> GAMGSGEPQSPSRRVFNPYTEFKEFSRKQIKDMEKMFKQYDAGRDGFIDLMELKLMMEKLGAPQTHLGLKNMIKEVDEDFD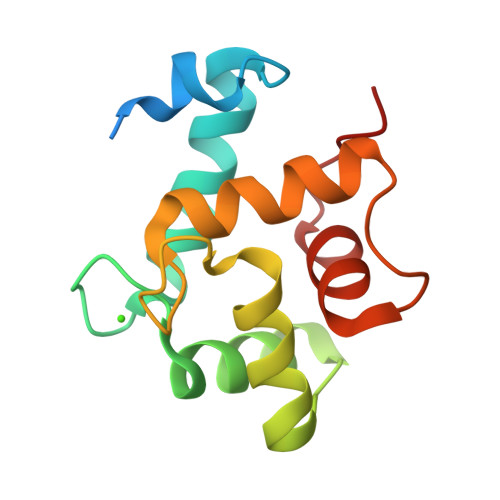SKLSFRAFLLIFRKAAAGELQEDSGLCVLARLSEIDVSS>[4x]ATRSPGVVISDDEPGYDLDLFCIPNHYAEDLERVFIPHGLIMDRTERLARDVMKEMGGHHIVALCVLKGGYKFFADLLDYIKALNRNSDRSIPMTVDFIRLKSYCNDQST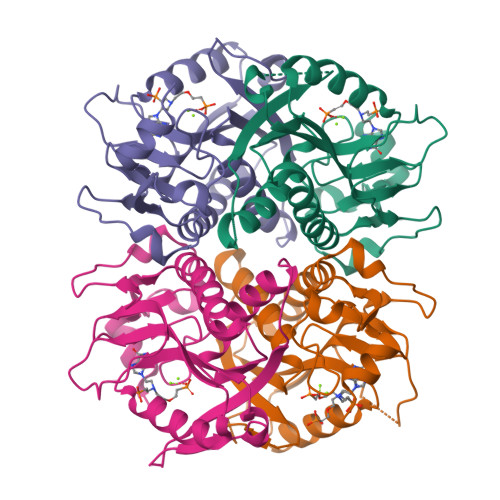GDIKVIGGDDLSTLTGKNVLIVEDIIDTGKTMQTLLSLVRQYNPKMVKVASLLVKRTPRSVGYKPDFVGFEIPDKFVVGYALDYNEYFRDLNHVCVISETGKAKYKA> GTRPNHTIYINNLNSKIKKDELKKSLHAIFSRFGQILDILVPRRRTPRGQAFVIFKEVSSATNALRSMQGFPFYDKPMAIQYAKTDR

The viral trans-activator of transcription (Tat) protein uses an archetypal arginine-rich motif (ARM) to recruit the host positive transcription elongation factor b (pTEFb) complex onto the viral trans-activation response (TAR) RNA, leading to activation of HIV transcription. Using yeast display and multiple rounds of selection, a new class of TAR-binding proteins (TBPs) was identified that bind TAR with nanomolar affinity. Here, we present four co-crystal structures of lab-evolved TAR-binding proteins (TBPs) in complex with HIV-1 TAR. Although it was hypothesized originally that each TBP variant would recognize TAR using fundamentally different modes of binding, we demonstrated here that each TBP binds TAR using a conserved subset of arginine-to-guanine interactions within a lab-evolved β2-β3 loop.

Although TBP6.3 contains four arginines, this variant exhibited 8.5-fold weaker binding than TBP6.7, which has three β2-β3 loop arginines. This observation prompted us to investigate TBP6.9 because it is identical to TBP6.7, except that position 48 is replaced by arginine. Unexpectedly, ITC revealed that TBP6.9 bound to TAR with a KD of 3.0 ± 0.3 nm and ΔΔG° of −0.4 kcal mol−1, indicating a nearly equivalent interaction energy compared with TBP6.7 and a slightly more favorable Krel of 0.6. However, the TAR-TBP6.9 co-crystal instead revealed only a subtle variation of the fundamental set of interactions first observed for three-arginine recognition of TAR by TBP6.7. Specifically, the Arg-48 guanidinium group of TBP6.9 interacts with the backbone at the pro-Sp oxygen of Gua36 in a manner analogous to Gln-48 of TBP6.7; simultaneously, Arg-47, Arg-49, and Arg-52 retained interactions with conserved major-groove guanine bases (Figs. 2B and 3 (E and H)). Collectively, the ITC results reveal that placement of arginine at position 48 can be favorable in the context of existing arginines at positions 47, 49, and 52—as seen for TBP6.9. We chose this variant because it contains four arginines and represents the tightest TAR binder in our ITC analysis. A second interaction is also shared among TBP6.7, TBP6.9, and TBP6.6. Each protein makes a hydrogen bond between Oγ1 of Thr-50 and Nε of Arg-52, stabilizing a favorable arginine rotamer for guanine recognition (Figs. 2B and 3 (E and F) and Fig. S3B). Additionally, Lys-50 and Lys-51 of Tat make phosphate-specific backbone interactions with TAR, whereas Arg-55 interacts with the backbone of 7SK. Such contacts are similar to Arg-52 of TBP6.3 and Arg-48 of TBP6.9.>[3x]MTTPPLLQLPVEVKKTELNGFWDTGAQITCIPEAFLKEEIPIGEAQIKTLHGTKLQSVYYLKFKVLGRKVEAEVTTSPFDYVIISPSDIPWYKPQPLELTVKLPVQDFKKELINKANINNEEKKQLAKLLDKYDVLWQQWENQVGHRKIPPHNIATGTVAPRPQRQYHINTKAKPSIQQVIDDLLKQGVLIKQTSVMNTPIYPVPKPDGKWRMVLDYRAVNKTVPLIGAQNQHSLGILTNLVRQKYKSTIDLSNGFWAHPITKDSQWITAFTWEGKQHVWTRLPQGFLNSPALFTADVVDLLKNIPGISVYVDDIYFSTETVSEHLKILEKVFKILLEAGYIVSLKKSALLRYEVTFLGFSITQTGRGLTSEFKDKIQNITSPRTLKELQSILGLFNFARNFVPNFSEIIKPLYSLISTAEGNNIKWTSEHTRYLEEIVSALNHAGNLEQRDNESPLVVKLNASPKTGYIRYYNKGGQKPIAYASHVFTNTELKFTPLEKLLVTMHKALIKAIDLALGQPIEVYSPIISMQKLQKTPLPERKALSTRWITWLSYLEDPRITFYYDKTLPDLKNVPETVTDKKPKMLPIIEYAAVFYTDGSAIRSPDKNKSHSSGMGIVHAVFKPELTIEHQWSIPLGDHTAQYAEISAVEFACKKANNISGPVLIVTDSDYVARSVNEELPFWRSNGFVNNKKKPLKHISKWKNISDSLLLKRDIIIVHEPGHKPSYTSIHTQGNNLADKLATQGSYTVNNI

Reverse transcriptases (RTs) use their DNA polymerase and RNase H activities to catalyze the conversion of single-stranded RNA to double-stranded DNA (dsDNA), a crucial process for the replication of retroviruses. Foamy viruses (FVs) have many characteristics that set them apart from OVs, including differences in the proliferation cycle and a different domain structure of the mature RT, which, in addition to POL and RH, harbors the N-terminal protease (PR) domain (PR-RT). Reverse transcriptases have two activities: DNA polymerase (POL) synthesizes DNA on DNA or RNA templates, whereas RNase H (RH) degrades the RNA strand of RNA/DNA hybrid intermediates. The structural and biophysical experiments showed that MFV PR-RT is a monomer upon binding to RNA/DNA and a dimer when it interacts with dsDNA.

To this aim, we used cryo-EM and obtained a 4.8-Å-resolution reconstruction of full-length MFV PR-RT in complex with a longer dsDNA comprising 22 bp and a 2-nt overhang at the 5′ end of the template strand (substrate 3) (see Materials and Methods for the sequence). The crystal structure of the PR-RT ΔRH–dsDNA complex was fitted into this cryo-EM reconstruction. The reconstruction corresponded well with the dimeric structure of the POL-connection portion of PR-RT ΔRH in complex with dsDNA. The cryo-EM data confirmed that the full-length MFV PR-RT forms dimers upon dsDNA binding. In the cryo-EM reconstruction, we did not observe any density for the protease domains, which indicates that they are more mobile than implied by the crystal structures. However, a density that corresponded to one of the RH domains was observed. The reconstruction does not clearly show which dimer subunit contributes this RH domain, but the C terminus of the connection domain of subunit A is located closer to the N terminus of this RH domain, so it is a more likely candidate. Interestingly, the RH domain interacts with the thumb subdomain of subunit B, which likely stabilizes the position of the RH domain. Moreover, the RH domain is in the vicinity of the dsDNA substrate, and charged residues Lys692, Lys694, Lys697, and His698 located in the basic protrusion are predicted to form contacts with the nucleic acid. In particular, the 22-bp dsDNA helix in the cryo-EM reconstruction shows only a very small bend of the DNA duplex.> MSKTAQKRLLKELQQLIKDSPPGIVAGPKSENNIFIWDCLIQGPPDTPYADGVFNAKLEFPKDYPLSPPKLTFTPSILHPNIYPNGEVCISILHSPGDDPNMYELAEERWSPVQSVEKILLSVMSMLSEP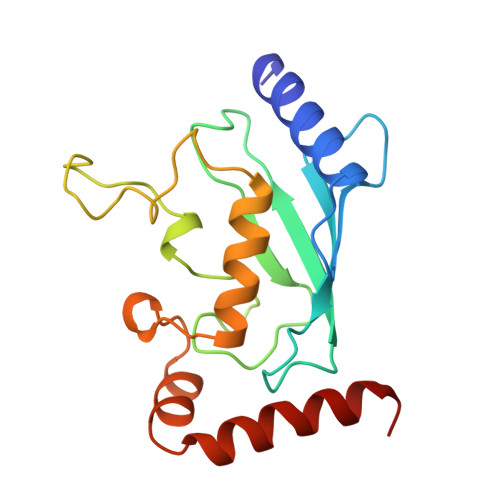NIESGANIDACILWRDNRPEFERQVKLSILKSLGF>MGDRSDHAKKLKTFLENLRRHLDRLDKHIKQLRDILSENPEDERVKDVIDLSERSVRIVKTVIKIFEDSVRKLLKQINKEAEELAKSPDPEDLKRAVELAEAVVRADPGSNLSKKALEIILRAAAELAKLPDPDALAAAARAASKVQQEQPGSNLAKAAQEIMRQASRAAEEAARRAKETLEKAEKDGDPETALKAVETVVKVARALNQIATMAGSEEAQERAARVASEAARLAERVLELAEKQGDPEVARRARELQEKVLDILLDILEQILQTATKIIDDANKLLEKLRRSERKDPKVVETYVELLKRHERLVKQLLEIAKAHAEAVEGGSLEHHHHHH[6x]

We develop a hierarchical approach to designing multi-component protein assemblies from two classes of modular building blocks: designed helical repeat proteins (DHRs) and helical bundle oligomers (HBs). We first rigidly fuse DHRs to HBs to generate a large library of oligomeric building blocks. We then generate assemblies with cyclic, dihedral, and point group symmetries from these building blocks using architecture guided rigid helical fusion with new software named WORMS. X-ray crystallography and cryo-electron microscopy characterization show that the hierarchical design approach can accurately generate a wide range of assemblies, including a 43 nm diameter icosahedral nanocage.

First, we explored the generation of C3, C4, and C5 assemblies with WORMS using heterodimer fusions. This resulted in head-to-tail cyclic ring structures dubbed “crowns” (Crn). We solved the structure of the C3_Crn-05 to 3.19 A resolution. The overall topology is as designed and the backbone geometry at each of the three junctions is close to the design model. A deviation at the tip of the undesigned heterodimeric HB is likely to due to crystal packing. Each of these structures experimentally verifies three distinct helical fusions (two HF, one WORMS) from the building block library that had not been characterized in isolation, confirming that the building blocks in the in silico library can have sufficient accuracy for subsequent building efforts.>MGSSHHHHHHSQDPIEGRAQVINTFDGVADYLQTYHKLPDNYITKSEAQALGWVASKGNLCDVAPGKSIGGDIFSNREGKLPGKSGRTWREADINYTCGFRNSD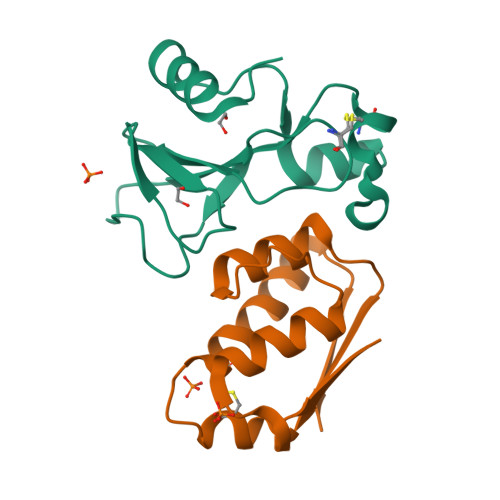RILYSSDWLIYKTTDHYQTFTKIR[2x];>[2x]MKKAVINGEQIRSISDLHQTLKKELALPEYYGENLDALWDALTGWVEYPLVLEWRQFEQCKQLTENGCESVLQVFREAKAEGADITIILS COPI mediates retrograde trafficking from the Golgi to the endoplasmic reticulum (ER) and within the Golgi stack, sorting transmembrane proteins bearing C-terminal KKxx or KxKxx motifs. The heptameric COPI complex (α/β/β'/γ/δ/ε/ζ) is recruited en bloc onto Golgi membranes (Hara-Kuge et al., 1994) but can be divided conceptually into two subcomplexes. The α/β'/ε B-subcomplex has been likened to clathrin because α-COP, β'-COP, and clathrin contain N-terminal WD-repeat (also referred to as β-propeller) domains and C-terminal α-solenoid domains and because recent studies have suggested that β'-COP, like clathrin, can form trimers. We demonstrate that N-terminal WD-repeat domains of α- and β'-COP directly bind dilysine motifs and establish the molecular bases for the interactions using X-ray crystallography, structure-directed mutagenesis, and isothermal titration calorimetry (ITC).

The first structure obtained was that of yeast β'1-304His6 in the presence of the CTFKKTN motif derived from yeast Wbp1 (Supplemental Experimental Procedures). This structure, solved at 1.8 Å resolution by SIRAS, showed that the WD-repeat domains pack one on top of the other in the lattice. The C-terminal His6 tag from one molecule reaches to the top surface of its neighbor, specifically occupying a charged surface patch. This structure suggested a potential binding site for short basic linear motifs, particularly highlighting the importance of a terminal carboxylate group and backbone carbonyl binding. The CTFKKTN peptide included in crystal trials was not visible in the density but was required for crystallization, likely forming weak interactions that facilitated crystal packing. Based on indirect evidence from structures, we predicted a D98A D117A mutant would abolish interaction with the -5 lysine. This prediction was based on the position of a histidine residue equivalent to the -5 lysine in the β'1-304His6 structure and of the symmetry copy K261 in the β'1-304 structure, both of which occupy the D98/D117 patch. In addition to the carboxylate group binding to the basic patch formed of R15/K17/R59, two carbonyl groups from the -2 and -3 positions in the motif backbone must fit into a groove formed by R59 and R101; the carbonyl group at the -4 position also likely contacts R101, as observed in the β'1-304His6 structure.

>[2x]MKLDIKKTFSNRSDRVKGIDFHPTEPWVLTTLYSGRVELWNYETQVEVRSIQVTETPVRAGKFIARKNWIIVGSDDFRIRVFNYNTGEKVVDFEAHPDYIRSIAVHPTKPYVLSGSDDLTVKLWNWENNWALEQTFEGHEHFVMCVAFNPKDPSTFASGCLDRTVKVWSLGQSTPNFTLTTGQERGVNYVDYYPLPDKPYMITASDDLTIKIWDYQTKSCVATLEGHMSNVSFAVFHPTLPIIISGSEDGTLKIWNSSTYKVEKTLNVGLERSWCIATHPTGRKNYIASGFDNGFTVLSLGNDEHHHHHH>GPHMLEREKIYQWINELSSPETRENALLELSKKRESVPDLAPMLWHSFGTIAALLQEIVNIYPSINPPTLTAHQSNRVCNALALLQCVASHPETRSAFLAAHIPLFLYPFLHTVSKTRPFEYLRLTSLGVIGALVKTDEQEVINFLLTTEIIPLCLRIMESGSELSKTVATFILQKILLDDTGLAYICQTYERFSHVAMILGKMVLQLSKEPSARLLKHVVRCYLRLSDNPRAREALRQCLPDQLKDTTFAQVLKDDTTTKRWLAQLVKNLQE[2x];>[2x]E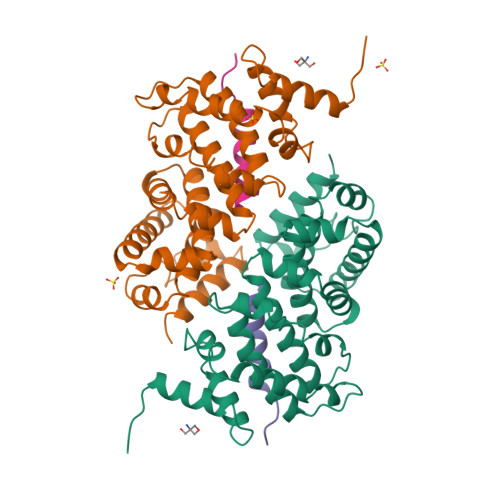GGIDSGMMLQLEKNLVDIVD> MA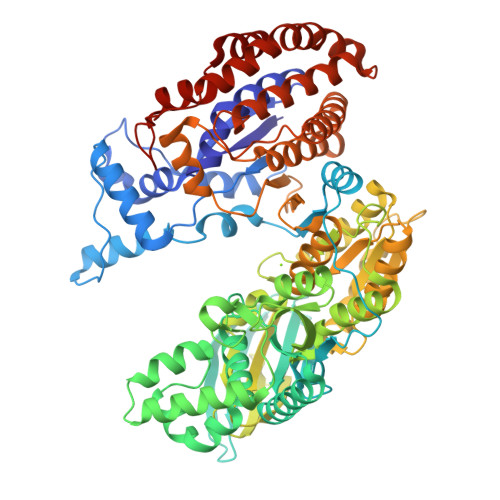KIIWTRTDEAPLLATYSLKPVVEAFAATAGIEVETRDISLAGRILAQFPERLTEDQKVGNALAELGELAKTPEANIIKLPNISASVPQLKAAIKELQDQGYDIPELPDNATTDEEKDILARYNAVKGSAVNPVLREGNSDRRAPIAVKNFVKKFPHRMGEWSADSKTNVATMDANDFRHNEKSIILDAADEVQIKHIAADGTETILKDSLKLLEGEVLDGTVLSAKALDAFLLEQVARAKAEGILFSAHLKATMMKVSDPIIFGHVVRAYFADVFAQYGEQLLAAGLNGENGLAAILSGLESLDNGEEIKAAFEKGLEDGPDLAMVNSARGITNLHVPSDVIVDASMPAMIRTSGHMWNKDDQEQDTLAIIPDSSYAGVYQTVIEDCRKNGAFDPTTMGTVPNVGLMAQKAEEYGSHDKTFRIEADGVVQVVSSNGDVLIEHDVEANDIWRACQVKDAPIQDWVKLAVTRSRLSGMPAVFWLDPERAHDRNLASLVEKYLADHDTEGLDIQILSPVEATQLSIDRIRRGEDTISVTGNVLRDYNTDLFPILELGTSAKMLSVVPLMAGGGLFETGAGGSAPKHVQQVQEENHLRWDSLGEFLALAESFRHELNNNGNTKAGVLADALDKATEKLLNEEKSPSRKVGEIDNRGSHFWLTKFWADELAAQTEDADLAATFAPVAEALNTGAADIDAALLAVQGGATDLGGYYSPNEEKLTNIMRPVAQFNEIVDALKK(1~{R},2~{R})-2,3-dihydro-1~{H}-indene-1,2-diol 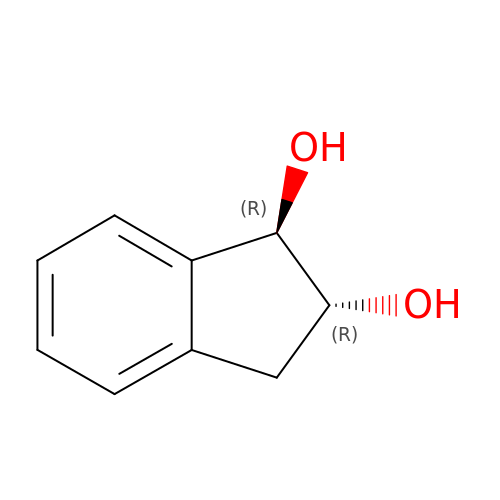| C9 H10 O2 | YKXXBEOXRPZVCC-RKDXNWHRSA-N>MTAIAPVITIDGPSGAGKGTLCKAMAEALQWHLLDSGAIYRVLALAALHHHVDVASEDALVPLASHLDVRFVSTNGNLEVILEGEDVSGEIRTQEVANAASQVAAFPRVREALLRRQRAFRELPGLIADGRDMGTVVFPDAPVKIFLDASSEERAHRRMLQLQEKGFSVNFERLLAEIKERD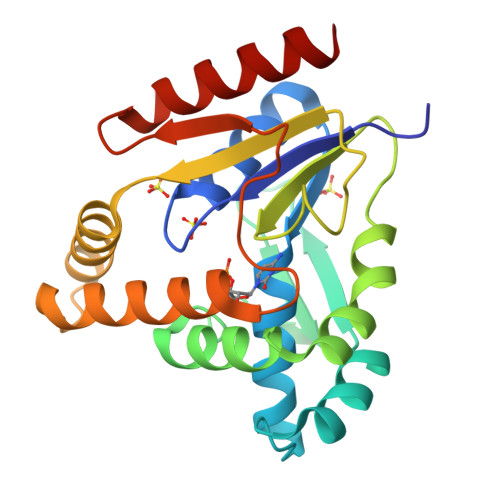DRDRNRAVAPLVPAADALVLDSTTLSIEQVIEKALQYARQKLALA[2x]> MGMEEIEHRTVEVNGIKMHVAEKGEGPVVLFLHGFPELWYSWRHQ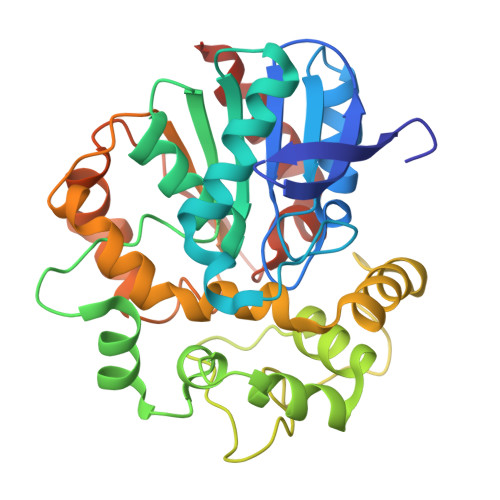ILALSSRGYRAVAPDLRGYGDTEAPVSISSYTGFHIVGDLIALIDLLGVDQVFLVAHDWGAIIGWYLCTFHPDRVKAYVCLSVPLLHRDPNIRTVDAMRAMYGDDYYICRFQKPGEMEAQMAEVGTEYVLKNILTTRKPGPPIFPKGEYGTGFNPDMPNSLPSWLTQDDLAYYVSKYEKTGFTGPLNYYRNMNLNWELTAPWSGGKIQVPVKFITGELDVVYTSLNMKEYIHGGGFKQDVPNLEEVIVQKNVAHFNNQEAAEEINNHIYDFIKKFLQHHHHHH>[2x]MALSWNEIRRKAIEFSKRWEDASDENSQAKPFLIDFFEVFGITNKRVATFEHAVKKFAKAHKEQSRGFVDLFWPGILLIEMKSRGKDLDKAYDQALDYFSGIAERDLPRYVLVCDFQRFRLTDLITKESVEFLLKDLYQNVRSFGFIAGYQTQVIKPQDPINIKAAERMGKLHDTLKLVGYEGHALELYLVRLLFCLFAEDTTIFEKSLFQEYIETKTLEDGSDLAHHINTLFYVLNTPEQKRLKNLDEHLAAFPYINGKLFEEPLPPAQFDKAMREALLDLCSLDWSRISPAIFGSLFQSIMDAKKRRNLGAHYTSEANILKLIKPLFLDELWVEFEKVKNNKNKLLAFHKKLRGLTFFDPACGCGNFLVITYRELRLLEIEVLRGLHRGGQQVLDIEHLIQINVDQFFGIEIEEFPAQIAQVALWLTDHQMNMKISDEFGNYFARIPLKSTPHILNANAL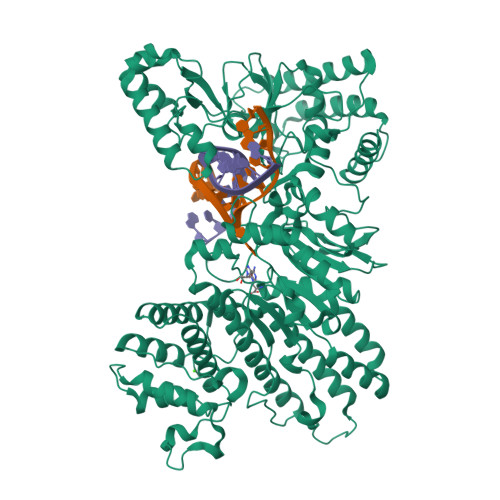QIDWNDVLEAKKCCFILGNPPFVGKSKQTPGQKADLLSVFGNLKSASDLDLVAAWYPKAAHYIQTNANIRCAFVSTNSITQGEQVSLLWPLLLSLGIKINFAHRTFSWTNEASGVAAVHCVIIGFGLKDSDEKIIYEYESINGEPLAIKAKNINPYLRDGVDVIACKRQQPISKLPSMRYGNKPTDDGNFLFTDEEKNQFITNEPSSEKYFRRFVGGDEFINNTSRWCLWLDGADISEIRAMPLVLARIKKVQEFRLKSSAKPTRQSASTPMKFFYISQPDTDYLLIPETSSENRQFIPIGFVDRNVISSNATYHIPSAEPLIFGLLSSTMHNCWMRNVGGRLESRYRYSASLVYNTFPWIQPNEKQSKAIEEAAFAILKARSNYPNESLAGLYDPKTMPSELLKAHQKLDKAVDSVYGFKGPNTEIARIAFLFETYQKMTSLLPPEKEIKKSKGKN>[2x]S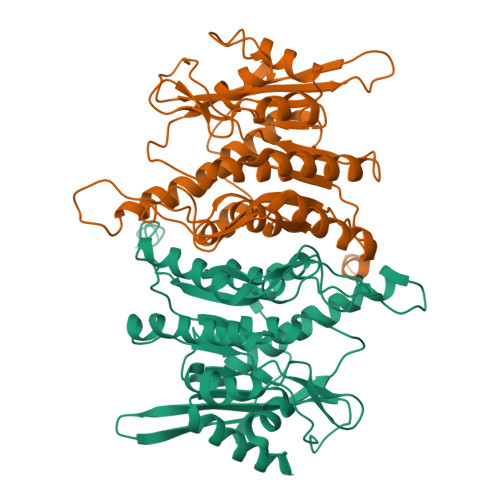YYHHHHHHHEGVRTMEEECRVLSIQSHVIRGYVGNRAATFPLQVLGFEIDAVNSVQFSNHTGYAHWKGQVLNSDELQELYEGLRLNNMNKYDYVLTGYTRDKSFLAMVVDIVQELKQQNPRLVYVCDPVLGDKWDGEGSMYVPEDLLPVYKEKVVPLADIITPNQFEAELLSGRKIHSQEEALRVMDMLHSMGPDTVVITSSDLPSPQGSNYLIVLGSQRRRNPAGSVVMERIRMDIRKVDAVFVGTGDLFAAMLLAWTHKHPNNLKVACEKTVSTLHHVLQRTIQCAKAQAGEGVRPSPMQLELRMVQSKRDIEDPEIVVQATVL> MSKIEKLSILGVRSFGPHHPETIAFNTPLTLIVGYNGSGKTTVIECLKYATTGELPPNSTRNGAFIHDPDLVGEKEVRAQVKLSFRSTIGESYVVTRNIQLLVQRNNKRTQKTLEGSLLLRNNGERTVISTRVAELDKL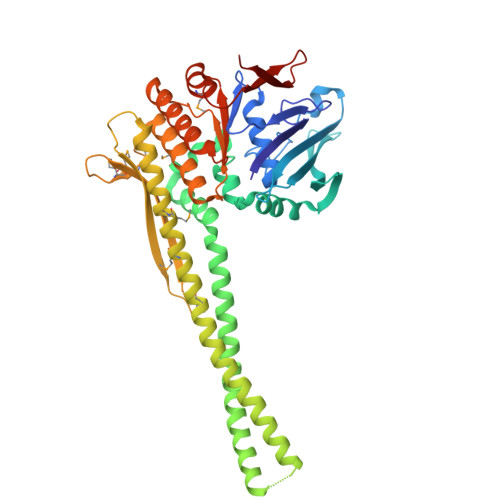VSEKLGVPPAILDAVIFCHQDDSLWPMSEPAALKKRFDEIFEAQKYTKVIENIRLLKKKKGDELKILKEREVQDKANKERAEKVDGGAGGAGGELDLKDAKAKYKETHIKVETTKAAIEDLGRGMAAVDHAIMQYHSKMMEQINRTIAELWQSTYQGTDIDTIQIRSDVESTTSSDSGTRRNYNYRVSMVKGDTEMDMRGRCSAGQKVLASIIIRLALAESFCANCGLIALDEPTTNLDSDNIRSLAESLHGIIKARQAQGNLQLIVITHDEEFLKYMQCSDFCDDFYRVKRDEKQNSVIVRESITRITE3-bromo-N'-[(1E)-(3,5-dibromo-2,4-dihydroxyphenyl)methylidene]benzohydrazide | C14 H9 Br3 N2 O3 | 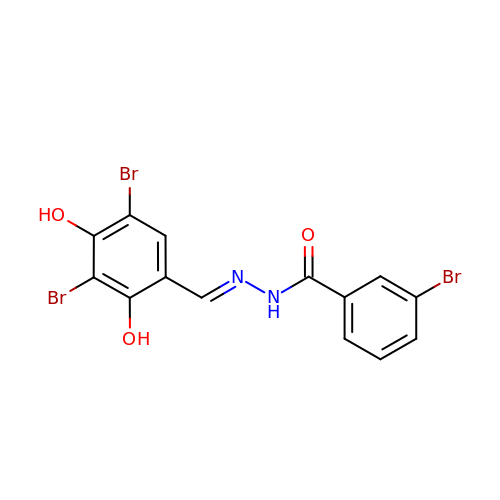VOWXAXNVAGLOGM-NGYBGAFCSA-N>TKHKERVMYYGKGDVFAYRTYLKPLTGVRTIPESPFSGRDHILFGVNVKISVGGTKLLTSFTKGDNSLVVATDSMKNFIQKHLASYTGTTI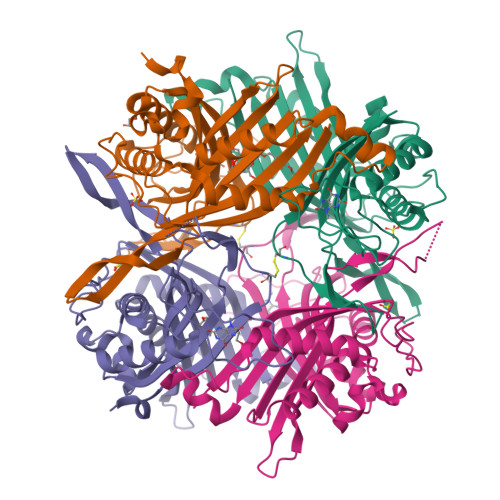EGFLEYVATSFLKKYSHIEKISLIGEEIPFETTFAVKNGNRAASELVFKKSRNEYATAYLNMVRNEDNTLNITEQQSGLAGLQLIKVSGNSFVGFIRDEYTTLPEDSNRPLFVYLNIKWKYKNTEDSFGTNPENYVAAEQIRDIATSVFHETETLSIQHLIYLIGRRILERFPQLQEVYFESQNHTWDKIVEEIPESEGKVYTEPCPPYGFQCFTVTQEDLPHENILMFSDEPDHKGALK[4x]> MVKAFWSALQIPELRQRVLFTLLVLAAYRLGAFIPTPGVDLDKIQEFLRTAQGGVFGIINLFSGGNFERFSIFALGIMPYITAAIIMQILVTVVPALEKLSKEGEEGRRIINQYTRIGGIALGAFQGFFLATAFLGAEGGRFLLPGWSPGPFFWFVVVVTQVAGIALLLWMAERITEYGIGNGTSLIIFAGIVVEWLPQILRTIGLIRTGEVNLVAFLFFLAFIVLAFAGMAAVQQAERRIPVQYARKVVGGRVYGGQATYIPIKLNAAGVIPIIFAAAILQIPIFLAAPFQDNPVLQGIANFFNPTRPSGLFIEVLLVILFTYVYTAVQFDPKRIAESLREYGGFIPGI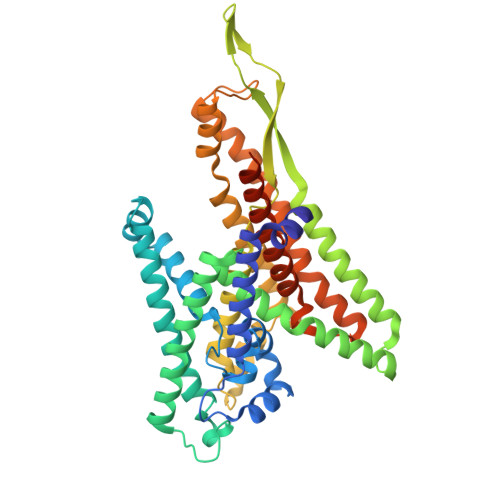RPGEPTVKFLEHIVSRLTLWGALFLGLVTLLPQIIQNLTGIHSIAFSGIGLLIVVGVALDTLRQVESQLMLRSYEGFLSRGRLRGRNRHHHHHH>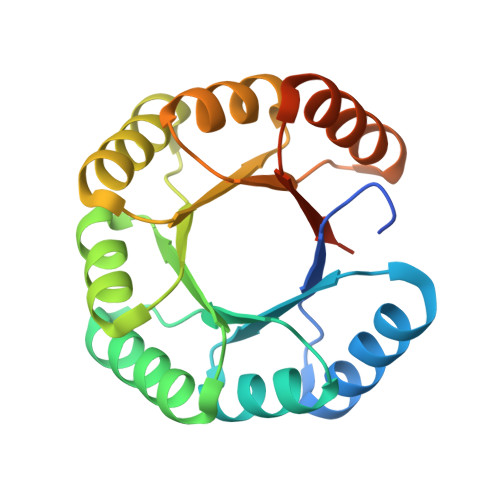 HHHHHHENLYFQSDIAIVDADNPADAIQQVKDLRKYGAKLIAYKSKSSEELKLALKAGADIAIVDADNPADAIQQVKDLRKYGAKLIAYKSKSSEELKLALKAGADIAIVDADNPADAIQQVKDLRKYGAKLIAYKSKSSEELKLALKAGADIAIVDADNPADAIQQVKDLRKYGAKLIAYKSKSSEELKLALKAG> DYKDDDDKGGGGSFRDCADVYQAGFNKSGIYTIYINNMPEPKKVFCNMDVNGGGWTVI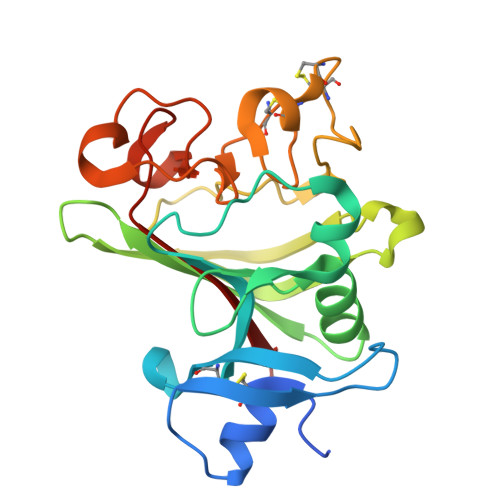QHREDGSLDFQRGWKEYKMGFGNPSGEYWLGNEFIFAITSQRQYMLRIELMDWEGNRAYSQYDRFHIGNEKQNYRLYLKGHTGTAGKQSSLILHGADFSTKDADNDNCMCKCALMLTGGWWFDACGPSNLNGMFYTAGQNHGKLNGIKWHYFKGPSYSLRSTTMMIRPLDF>[8x]GPHMSGSRKFFVGGNWKMNGSRDDNDKLLKLLSEAHFDDNTEVLIAPPSVFLHEIRKSLKKEIHVAAQNCYKVSKGAFTGEISPAMIRDIGCDWVILG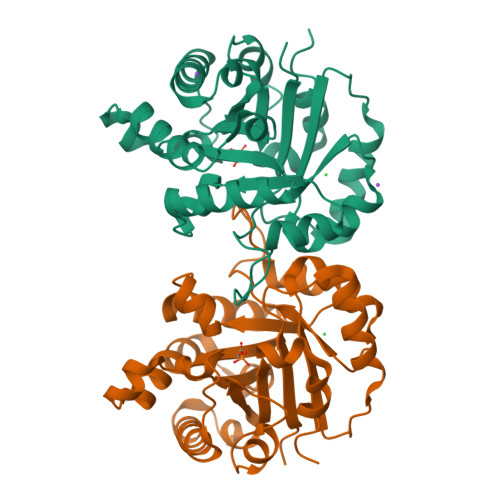HSERRNIFGESDELIAEKVQHALAEGLSVIACIGETLSERESNKTEEVCVRQLKAIANKIKSADEWKRVVVAYEPVWAIGTGKVATPQQAQEVHNFLRKWFKTNAPNGVDEKIRIIYGGSVTAANCKELAQQHDVDGFLVGGASLKPEFTEICKARQR> GSHMTRETERFPAREFQRDLLDWFARERRDLPWRKDRDPYKVWVSEVMLQQTRVETVIPYFEQFIDRFPTLEALADADEDEVLKAWEGLGYYSRVRNLHAAVKEVKTRYGGKVPDDPDEFSRLKGVGPYTVGAVLSLAYGVPEPAVDGNVMRVLSRLFLVTDDIAKCSTRKRFEQIVREIMAYENPGAFNEALIELGALVCTPRRPSCLLCPVQAYCQAFAEGVAEELPVKMKKTAVKQVPLAVAVLADDEGRVLIRKRDSTGLLANLWEFPSCETDGADGKEKLEQMVGEQYGLQVELTEP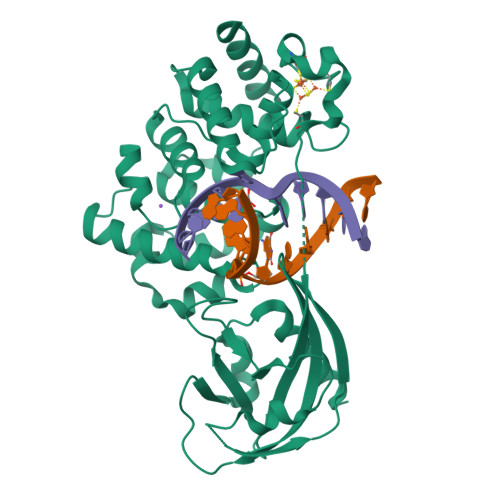IVSFEHAFSHLVWQLTVFPGRLVHGGPVEEPYRLAPEDELKAYAFPVSHQRVWREYKEWASGVRPPP>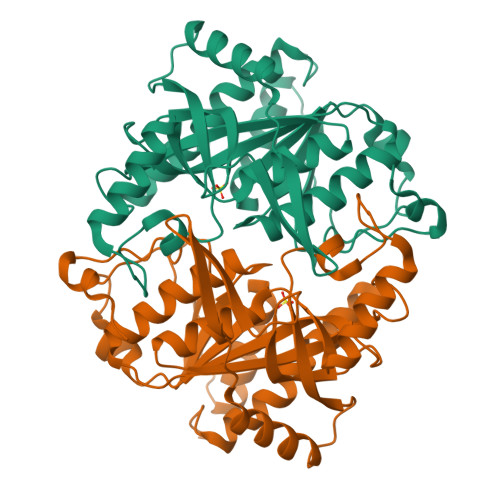MATVQPIVNSHLSELDEDVFHHFGFTTKSFDFKEKFGDVKFVCVCGSSGRIHNFAISMAKLAGLALPVENIAGSHARFVLYKVDHILFADHGMGIPSALIMLHEVTKLLHYAGCKDVLFIRLGTSGGLGVKPGTIVLSDRCVNTKLEPYNELCILGKPVRRQTIVDLNTVNELKKLSENLSLECSVVVGGTIAANDFYEEQGRLDGSICTFSKEEKLAFLQSAYEHGIRNMEMEGTAITSHCYLTGHRAILVCVTAVNRLEGDQITISTDEFTLFAQRPGQLVGEYLKRNNGIIVR[4x]> PPKTPRNVFFPWQVFSVHRTGAFLERRRVALKVPVNLTKFEIQSYLEKIYGARVLKVSTLIVVPRRRRDIFGPRPSMRYYRVGCTFKK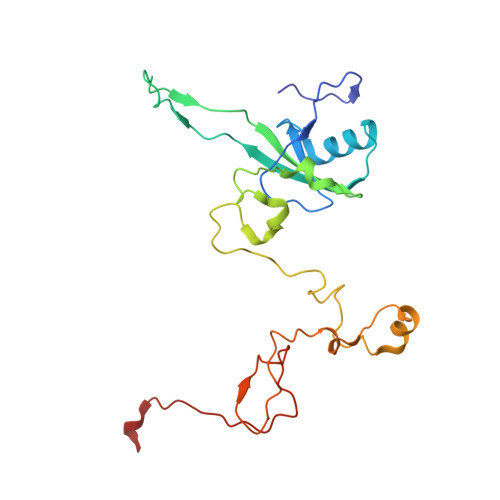AIVTLEDGVPDAVKMLRSSIELAKNPDITKHNLTYSGRVRAFKPPSAAQRWEMGESKYAWRLPIPNLLAGDEMQLNPALRIDESTTQMFPDFSKPFFHNAHFNFSWKPEEVPFQQTVKLDITPWRR> GAGCAGACGTG;> ACTCCACTCA;> CAAGT;> TCTGAGTGGCGTCTGC

In this work, we exhaustively probe the ability of all 36 immobile HJ sequences to form DNA crystals in two different designed systems. Three separate self-assembling DNA crystal systems are described in this report: the “4 × 5” and “4 × 6” designs (collectively referred to as the 4 × N systems), and a third construct with a “scrambled” sequence variant of the 4 × 6 lattices. Self-assembly was mediated by three constituent oligonucleotides: (S1) containing four sequence repeats of either 5 or 6 bases; (S2) composed of 21 bases containing complementary regions to both (S1); and (S3) which forms the second junction crossover. The HJ serves as the fundamental component at the core of each unit, and the ultimate assembly of the full lattice is facilitated by the complementary 2-base sticky ends that tail each duplex.

The 4 × 5 system robustly crystallized with 75% of the junctions, and we obtained crystals in all but 9 of 36 sequences. Of the resulting structures, 18 exhibited P32 symmetry with average cell dimensions a = b = 68.85 Å c = 60.09 Å, with only nine retaining the original P3221 symmetry with average cell edges a = b = 68.17 Å c = 60.60 Å. Although the cell parameters between the two symmetries were virtually indistinguishable, the differences between the periodicity of the lattices is dramatic, with vastly different cavity sizes. The P32 channels were treated as a hexagonal prism with 6.4 nm along each edge and a height measured from the top to the bottom of each block along with the average c-axis = 6.0 nm, with a resulting volume of ~639 nm3, a nearly 27-fold increase in cavity size relative to the P3221 lattices.>[4x]MSVRIVDVREITKPISSPIRNAY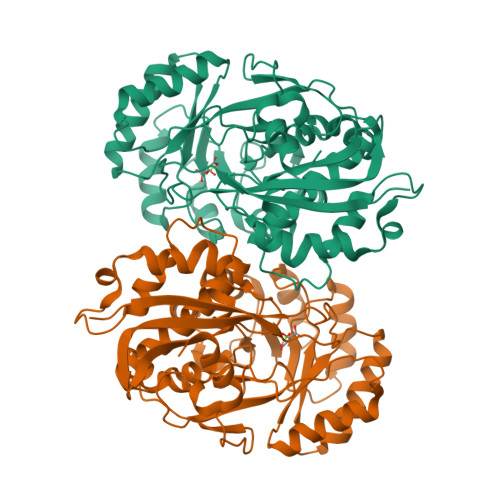IDFTKMTTSLVAVVTDVVREGKRVVGYGFNSNGRYGQGGLIRERFASRILEADPKKLLNEAGDNLDPDKVWAAMMINEKPGGHGERSVAVGTIDMAVWDAVAKIAGKPLFRLLAERHGVKANPRVFVYAAGGYYYPGKGLSMLRGEMRGYLDRGYNVVKMAIGGAPIEEDRMRIEAVLEEIGKDAQLAVDANGRFNLETGIAYAKMLRDYPLFWYEEVGDPLDYALQAALAEFYPGPMATGENLFSHQDARNLLRYGGMRPDRDWLQFDCALSYGLCEYQRTLEVLKTHGWSPSRCIPHGGHQMSLNIAAGLGLGGNESYPDLFQPYGGFPDGVRVENGHITMPDLPGIGFEGKSDLYKEMKALAE> MGQALGIKSCDFQAARNNEEHHTKALSSRRLFVRRGQPFTIILYFRAPVRAFLPALKKVALTAQTGEQPSKINRTQATFPISSLGDRKWWSAVVEERDAQSWTISVTTPADAVIGHYSLLLQVSGRKQLLLGQFTLLFNPWNREDAVFLKNEAQRMEYLLNQNGLIYLGTADCIQAESWDFGQFEGDVIDLSLRLLSKDKQVEKWSQPVHVARVLGA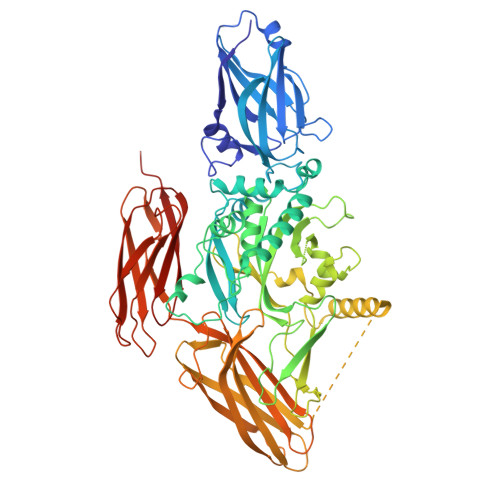LLHFLKEQRVLPTPQTQATQEGALLNKRRGSVPILRQWLTGRGRPVYDGQAWVLAAVACTVLRCLGIPARVVTTFASAQGTGGRLLIDEYYNEEGLQNGEGQRGRIWIFQTSTECWMTRPALPQGYDGWQILHPSAPNGGGVLGSCDLVPVRAVKEGTLGLTPAVSDLFAAINASCVVWKCCEDGTLELTDSNTKYVGNNISTKGVGSDRCEDITQNYKYPEGSLQEKEVLERVEKEKMEREKDNGIRPPSLETASPLYLLLKAPSSLPLRGDAQISVTLVNHSEQEKAVQLAIGVQAVHYNGVLAAKLWRKKLHLTLSANLEKIITIGLFFSNFERNPPENTFLRLTAMATHSESNLSCFAQEDIAICRPHLAIKMPEKAEQYQPLTASVSLQNSLDAPMEDCVISILGRGLIHRERSYRFRSVWPENTMCAKFQFTPTHVGLQRLTVEVDCNMFQNLTNYKSVTVVAPELSA> MDPDELPLDEHCERLPYDASKWEFPRDRLKLGKPLGRGAFGQVIEADAFGIDKTATCRTVAVKMLKEGATHSEHRALMSELKILIHIGHHLNVVNLLGACTKPGGPLMVIVEFCKFGNLSTYLRSKRNEFVPYKTKGARFRQGKDYVGAIPVD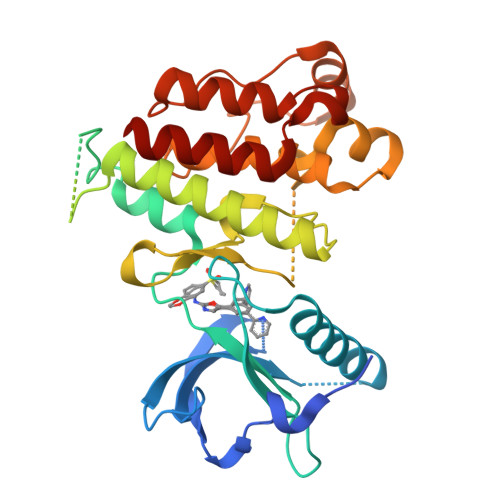LKRRLDSITSSQSSASSGFVEEKSLSDVEEEEAPEDLYKDFLTLEHLICYSFQVAKGMEFLASRKCIHRDLAARNILLSEKNVVKICDFGLARDIYKDPDYVRKGDARLPLKWMAPETIFDRVYTIQSDVWSFGVLLWEIFSLGASPYPGVKIDEEFCRRLKEGTRMRAPDYTTPEMYQTMLDCWHGEPSQRPTFSELVEHLGNLLQANAQQD>[6x]MHHHHHHMANCERTFIAIKPDGVQRGLVGEIIKRFEQKGFRLVGLKFMQASEDLLKEHYVDLKDRPFFAGLVKYMHSGPVVAMVWEGLNVVKTGRVMLGESNPADSKPGTIRGD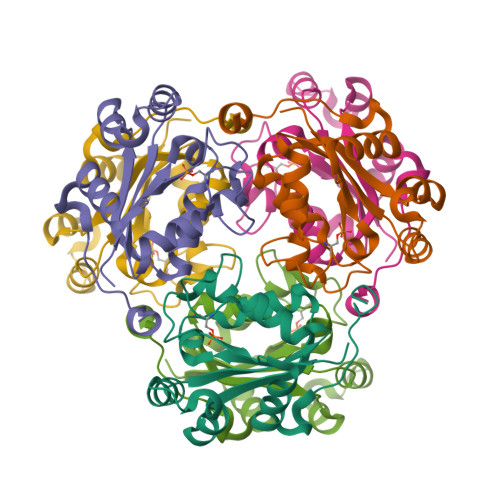FCIQVGRNIIHGSDSVESAEKEIGLWFHPEELVDYTSCAQNWIYE> MRETDEEPEEPGRRGSFVEMVDNLRGKSGQGYYVEMTVGSPPQTLNILVDTGSSNFAVGAAPHPFLHRYYQRQLSSTYRDLRKGVYVPYTQGKWEGELGTDLVSIPHGPNVTVRANIAAITESDKFFINGSNWEGILGLAYAEIARPDDSLEPFFDSLVKQTHVPNLFSLQLCGAGFPLNQSEVLASVGGSMIIGGIDHSLYTGSLWYTPIRREWYYEVIIVRVEINGQDLKMDCKEYNYDKSIVDSGTTNLRLPKKVFEAAVKSIKAASSTEKFPDGFWLGEQLVCWQAGTTPWNIFPVISLYLMGEVTNQSFRITILPQQYLRPVEDVATSQDDCYKFAISQSSTGTVMGAVIMEGFYVVFDRARKRIGFAVSACHVHDEFRT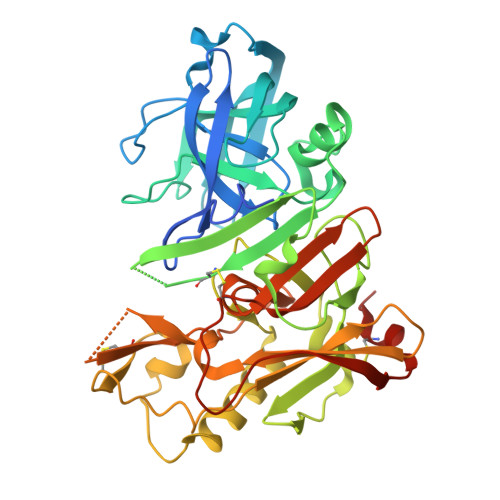AAVEGPFVTLDMEDCGYNIPQTDEST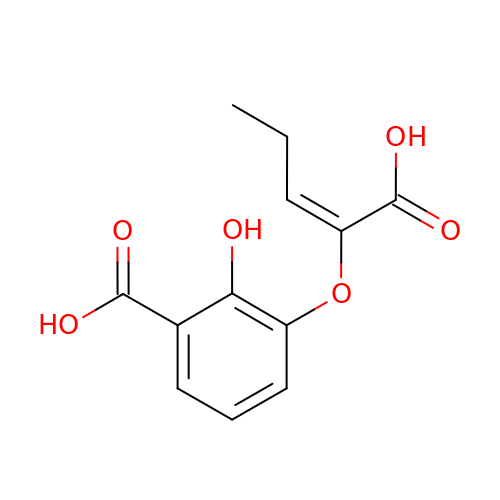3-{[(1Z)-1-carboxybut-1-en-1-yl]oxy}-2-hydroxybenzoic acid | C12 H12 O6 | NMNSLXCRMLAOLT-WTKPLQERSA-N Dystrophin is a large (427 kD) multidomain protein expressed in skeletal and cardiac muscle where it binds to the dystrophin-associated glycoprotein (DAG) complex of the plasma membrane and to F-actin connecting the cytoskeleton to the membrane. Utrophin (Utr), the 395 kD autosomal homologue of Dys is widely expressed in non muscle tissues (reviewed) but is restricted to the myotendinous and neuromuscular junctions of differentiated muscle and is located at the sarcolemma of developing fetal muscle. Dys and Utr potentially act as cellular biomechanical shock-absorbers limiting damage to the plasma membrane with the spectrin repeat domains acting as spring units by undergoing force-induced unfolding. Dys and Utr-SR1 adopt the canonical spectrin repeat fold comprising a triple helical bundle displaying an approximately cylindrical structure of overall dimensions ∼60 Å length and ∼9 Å radius (between backbone atoms).

Additionally we have determined the structure of a six amino acid longer version of the Utr-SR1 protein (amino acids 308–430, Utr-SR1-L) produced as a result of presumed proteolysis during crystallization experiments of an Utr N-terminal two spectrin repeat protein construct (Utr-SR1-SR2; 308–537). SDS-PAGE analysis of dissolved Utr-SR1-L crystals showed they contained a single 15 kD species. The Utr-SR1-L crystals are isomorphous with Utr-SR1 with insufficient space in the crystal lattice for the complete two domain SR1–SR2 structure. For the longer Utr-SR1-L structure we observe the start of the heptad repeat phasing for the next repeat domain SR2. The very C-terminus of Utr-SR1-L, corresponding to the N-terminus of SR2 helix A’, has rotated about the C-A’ helix axis, relative to homologous structures, forming an anti-parallel inter-helix interaction with a crystallographically-related molecule. It is likely that this rotation is a result of crystal packing rather than a reorientation of SR2 relative to SR1 although variation in domain orientation is observed for this protein family; a complete Dys/Utr-SR1-SR2 structure is required to conclusively define the inter-domain orientation.

>DMDLDSYQIALEEVLTWLLSAEDTFQEQDDISDDVEDVKEQFATHETFMMELSAHQSSVGSVLQAGNQLMTQGTLSDEEEFEIQEQMTLLNARWEALRVESMERQSRLHDALMELQKKQLQQL[2x]> ALVKEEIQAKEYLENLNKELAKRTNVETEAAWAYGSNITDENEKKKNEISAELA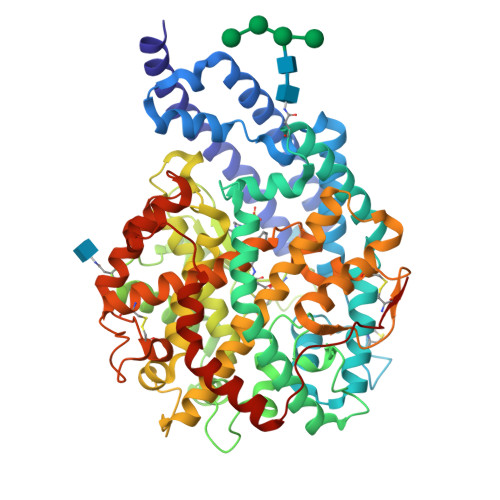KFMKEVASDTTKFQWRSYQSEDLKRQFKALTKLGYAALPEDDYAELLDTLSAMESNFAKVKVCDYKDSTKCDLALDPEIEEVISKSRDHEELAYYWREFYDKAGTAVRSQFERYVELNTKAAKLNNFTSGAEAWLDEYEDDTFEQQLEDIFADIRPLYQQIHGYVRFRLRKHYGDAVVSETGPIPMHLLGNMWAQQWSEIADIVSPFPEKPLVDVSAEMEKQGYTPLKMFQMGDDFFTSMNLTKLPQDFWDKSIIEKPTDGRDLVCHASAWDFYLTDDVRIKQCTRVTQDQLFTVHHELGHIQYFLQYQHQPFVYRTGANPGFHEAVGDVLSLSVSTPKHLEKIGLLKDYVRDDEARINQLFLTALDKIVFLPFAFTMDKYRWSLFRGEVDKANWNCAFWKLRDEYSGIEPPVVRSEKDFDAPAKYHISADVEYLRYLVSFIIQFQFYKSACIKAGQYDPDNVELPLDNCDIYGSAAAGAAFHNMLSMGASKPWPDALEAFNGERIMSGKAIAEYFEPLRVWLEAENIKNNVHIGWTTSNKCVSS> SMNYFVGNSLGVNLTGIEKAIINRLNLFKEMGRPAQCVFLSWNRYLYRNAQNYITSSDYINMYDFFQEATYLERNEPFDWLSYWTDECHYTLKHVENSHDFRIYDQERFLMYAHFQDPKYRILDYVNHFDSQRRKVKRDFYDVRGFLSCSRILVDKQQTLCEFFYNPEGDTKLEKYFSYKDGKPEVQKIIVYYANKQYFFNNETELGAFFIKQLYQHGDLFFSDRNVYTAPIFNLTPESIPVVAVLHSTHIKNIDALDSSPFKNVYKAMFENLSRYRAIIVSTEQQKLDVEKRINHTIPVVNIPVGYSETIDTPVQTLDQRSVKLISVARYSPEKQLHQQIELIKRLVSYVPKIELHMYGFGSESKKLNELIQKYGLENHVYLRGFLSNLDQEYSDAYLSLITSNMEGFSLALLESLAHGVPVISYDIKYGPNELITSDFNGYLITKNDEDALFDK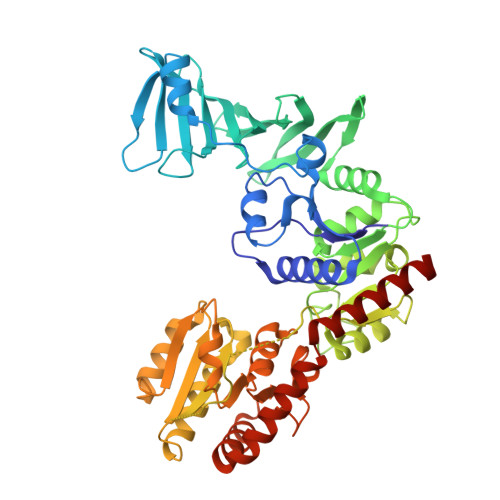VKYVIDHPEVQQRLSKGSLAKAQQYSKASLIKQWDQFVRLILEHHHHHH> FNKIKDSVKQKIDSMGDKGTYGVSASHPLAVEEGMKVLK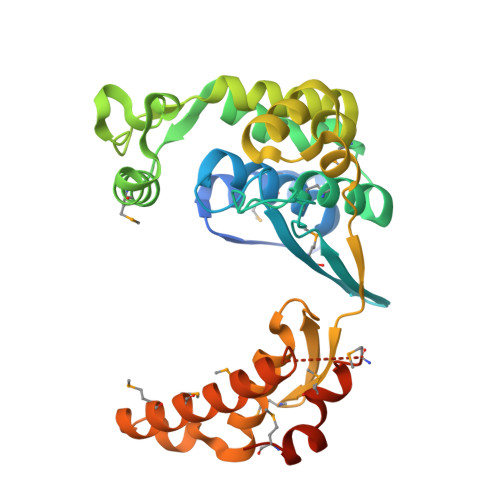NGGSAVDAAIVVSYVLGVVELHASGIGGGGGMLIISKDKETFIDYRETTPYFTGNQKPHIGVPGFVAGMEYIHDNYGSLPMGELLQPAINYAEKGFKVDDSLTMRLDLAKPRIYSDKLSIFYPNGEPIETGETLIQTDLARTLKKIQKEGAKGFYEGGVARAISKTAKISLEDIKGYKVEVRKPVKGNYMGYDVYTAPPPFSGVTLLQMLKLAEKKEVYKDVDHTATYMSKMEEISRIAYQDRKKNLGDPNYVNMDPNKMVSDKYISTMKNENGDALSEAEHES> MQIITAEDYRLYGGLKRPELESGVEVMITAANALITSLLGMDDADAVDQ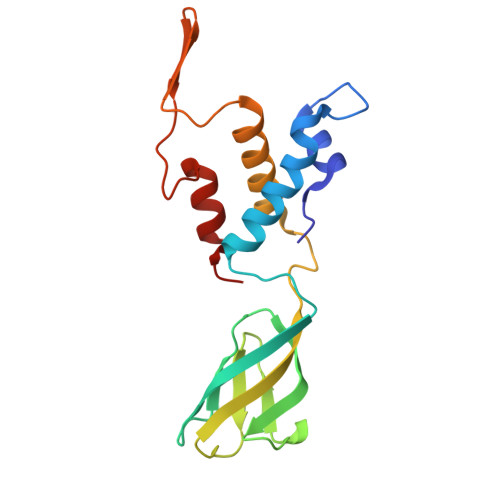LITTKPTRKKYFLSSPSATSVTKMTINDKEIDPEQYKLYSDGVILLKFNPPEGYMDVEYTQGGFNPMPEDLKLAACMLVDHWHKQDYRQARTIGGETVTFNNTKSGIPEHIRTIIEVYRRV Curli fibers are a major component of the extracellular matrix of Gram-negative bacteria and are expressed under biofilm forming conditions where they fulfill a scaffolding and cementing role in the extracellular milieu to reinforce the bacterial community. Here we combine extensive AlphaFold2 modelling and cryo-electron transmission microscopy to propose an atomic model of curli protofibrils, and their higher modes of organization. All models share a similar β-solenoid architecture, wherein curlin repeats fold into strand-β-arc-strand motifs that stack vertically to produce an in-register double, parallel β-sheet structure with a single strand stagger (i.e., 2.4 Å) between both sheets. Our results show that the curli protofibril consists of a highly regular supermolecular β-solenoid with an absent or negligible helical twist.

As a representative structure of CS-class CsgA monomers we discuss the AF2 model of A0A0E3UX01 (pLDDT=93.68), which has 15 curlin repeats and an additional half repeat at the C-terminus (hereafter referred to as R15.5). AF2 predicts a highly regular (the average main chain RMSD between consecutive repeats is 0.18 ± 0.02 Å), left-handed β-solenoid with a negligible twist (average main chain RMSD of top 5 AF2 models: 0.48 ± 0.38 Å). A transversal, on-axis view provides further insight into the structural nature of the steric zipper, which comprises a central hydrophobic core composed of the Ψ1 and Ψ2 residues in motif a and b, flanked on either side by a glutamine (Gln), followed by an asparagine (Asn), forming the pseudo centrosymmetric core predicted based on motif a and b sequence features. However, R15.5 has an uneven number of strands (i.e., 31), resulting in a motif a overhang both at N and C-termini. Rather, a proper match of two motif a overhangs across a dimer interface would require a fiber consisting of consecutive head-head—tail–tail interactions, or head-to-tail interactions with a twofold screw, i.e., 180° rotation of consecutive subunits along the fiber long axis. Disulfide formation of Cys residues introduced across the R15.5 interface occurred in accordance with a 21 screw axis, and also de novo prediction by AF2 showed a head-to-tail 21 screw in the subunit-subunit interface. For this we selected R15.5 due to its high Asp and Glu content (20%; pI = 2.98) leading us to hypothesize that R15.5 protofibrils would be less prone to tangle up because of repulsive electrostatics. The R15.5 side-view is nearly identical to the side-view of E. coli curli, suggesting that ex vivo curli and in vitro R15.5 fibrils are structurally equivalent at the fold level and essentially in agreement with AF2 predictions. The docking of an R15.5 AF2 model shows good agreement between the experimental cryoEM volume and the predicted β-solenoidal architecture. The reported Refine3D volume therefore represents a map that is longitudinally averaged over the curlin repeats.

>[3x]QGTTSSATTSQTGNTNTAVIDQVGGLNNSAEASQAGDGNVATVTQAEGMDNAVYIDQVGLTNTATVLQEGGLDNDADVDQDGDLNVAYIWQNLGEDNDADIDQDGTLNDAAIEQDGGEDNDADIDQDGSENAAYVGQTGGEDNDADIDQDGTFNNAYIGQFGGEDNEADLDQDGDANYAAILQDGGEDNDADIDQDGTNNWAETNQIQGNDNDVEVDQDGSDNIAEVWQMHGEDNEANVDQDGDLNNAYILQEGGMNNLADVHQNGVSNTAEIYQYGGMDNEAYLIQDGDMHTGVITQSGDGANYAELNQMGLMNTGSITQDGMGNSAITSQGGSMNMSTVTQSGTGNISLVNQHGGHHHHHH> GTTGMPQYSTFHSENRDWTFNHLTVHRRTGAVYVGAINRVYKLTGNLTIQVAHKTGPEEDNKACYPPLIVQPCSEVLTLTNNVNKLLIIDYSENRLLACGSLYQGVCKLLRLDDLFILVEPSHKKEHYLSSVNKTGTMYGVIVRSEGEDGKLFIGTAVDGKQDYFPTLSSRKLPRDPESSAMLDYELHSDFVSSLIKIPSDTLALVSHFDIFYIYGFASGGFVYFLTVQPETPDGMAINSAGDLFYTSRIVRLCKDDPKFHSYVSLPFGCTRAGVEYRLLQAAYLAKPGEALAQAFNISSDEDVLFAIFSKGQKQYHHPPDDSALCAFPIRAINLQIKERLQSCYHGEGNLELNWLLGKDVQCTKAPVPIDDNFCGLDINQPLG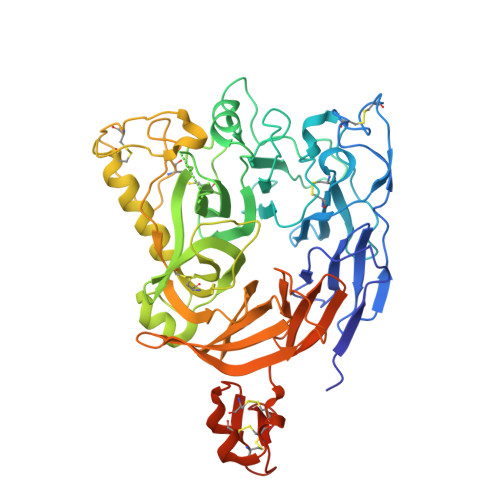GSTPVEGLTLYTTSRDRLTSVASYVYNGYSVVFVGTKSGKLKKIRADGPPHGGVQYEMVSVFKDGSPILRDMAFSINQLYLYVMSERQVTRVPVESCEQYTTCGECLSSGDPHCGWCALHNMCSRRDKCQRAWEANRFAASISQCMSSRENLYFQ> GAGCAGACCCGA;> CGGGACTCA;>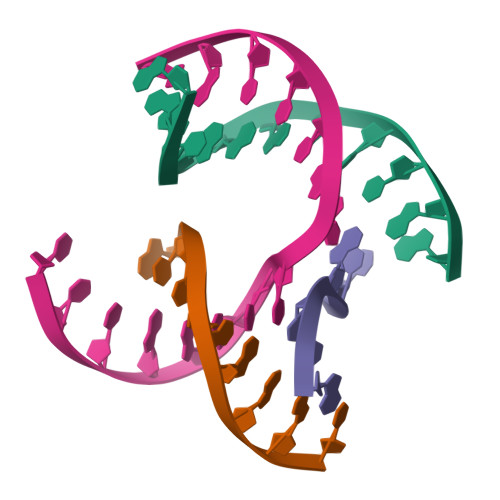 TCGCCG;> TCTGAGTCGGTCTGC> MSISKDSRIAIIGAGPAGLAAGMYLEQAGFHDYTILERTDHVGGKCHSPNYH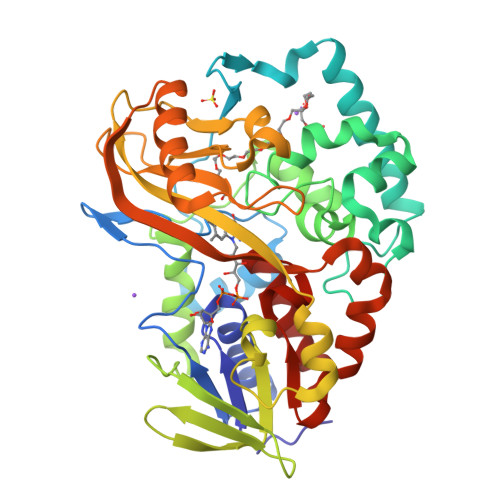GRRYEMGAIMGVPSYDTIQEIMDRTGDKVDGPKLRREFLHEDGEIYVPEKDPVRGPQVMAAVQKLGQLLATKYQGYDANGHYNKVHEDLMLPFDEFLALNGCEAARDLWINPFTAFGYGHFDNVPAAYVLKYLDFVTMMSFAKGDLWTWADGTQAMFEHLNATLEHPAERNVDITRITREDGKVHIHTTDWDRESDVLVLTVPLEKFLDYSDADDDEREYFSKIIHQQYMVDACLVKEYPTISGYVPDNMRPERLGHVMVYYHRWADDPHQIITTYLLRNHPDYADKTQEECRQMVLDDMETFGHPVEKIIEEQTWYYFPHVSSEDYKAGWYEKVEGMQGRRNTFYAGEIMSFGNFDEVCHYSKDLVTRFFV> MLPKRRRARVGSPSGDAASSTPPSTRFPGVAIYLVEPRMGRSRRAFLTGLARS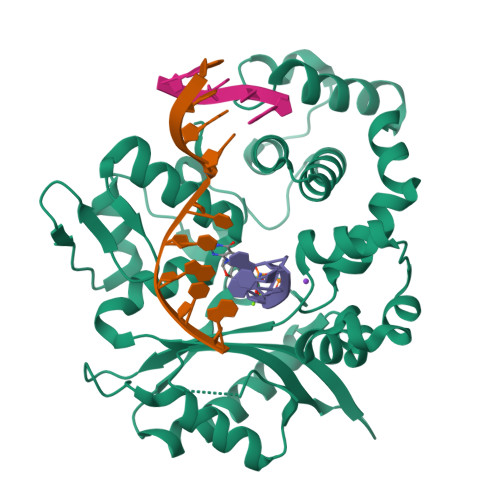KGFRVLDACSSEATHVVMEETSAEEAVSWQERRMAAAPPGCTPPALLDISWLTESLGAGQPVPVECRHRLEVAGPRKGPLSPAWMPAYACQRPTPLTHHNTGLSEALEILAEAAGFEGSEGRLLTFCRAASVLKALPSPVTTLSQLQGLPHFGEHSSRVVQELLEHGVCEEVERVRRSERYQTMKLFTQIFGVGVKTADRWYREGLRTLDDLREQPQKLTQQQKAGLQHHQDLSTPVLRSDVDALQQVVEEAVGQALPGATVTLTGGFRRGKLQGHDVDFLITHPKEGQEAGLLPRVMCRLQDQGLILYHQHQHSCCESPTRLAQQSHMDAFERSFCIFRLPQPGSWKAVRVDLVVAPVSQFPFALLGWTGSALFARELRRFSRKEKGLWLNSHGLFDPEQKTFFQAASEEDIFRHLGLEYLPPEQRNA> AI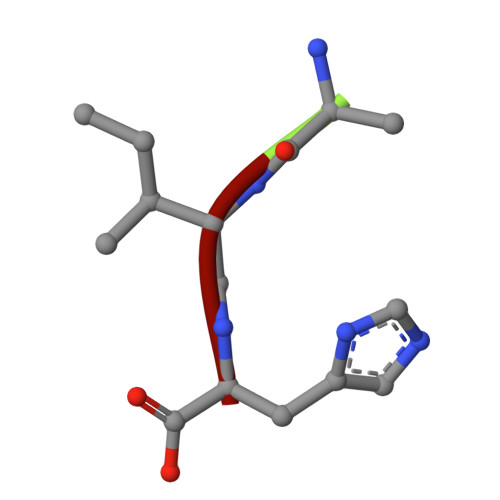H>[2x]IAPLVGYAIGAAAISAVGGIGVGWTLREFEVVGSDDPAEGLTPDVLRNQLSDSVVKRKSNNQSTMVDNQNILDGVEHTAYTEAKIAAIEELNAGSSESAVLSAANSAIDSYETTVRTNFYKSWNETVRELEAMTQTVIAHADVGLSYITDFGDPRFGNLASGTSPNTLKDTTVSMPDGTNFTLLTFRHNTGWDSGNAAYSVVEYNPKEVVTSTNSNTYNTVDGTQYMKFSEWNAVETEMDTVFQNVRNGISTWVTNVYGDVQSGAIEISDLVTPRERATMMAQEEGMSQAIADLIALNVPVDAEREATITIQDTGATLPGTFALTDSSDGPLSAGQTYDPSTFSGDVYFTADMSLVEGPWDAINSGVDGGTITITSEPYEGTAIEVTTVESETVSVPAADWTDNGDGTWSYDASGDLETTITNVDSARFVSTATETTYDTLQLKGAFTVDKLVNKQSGEEVSSTSFTSSEPQTDSNYITQDEWDQLEQQNKELIEKYEQSQSGGGLDLGGLD

Haloarchaeal pleomorphic viruses (HRPVs) infect archaeal hosts living in hypersaline environments. The virions contain two major protein species, a spike protein (VP4 and VP4-like proteins) protruding from the membrane surface and a smaller membrane associated protein (VP3 and VP3-like proteins) residing mostly inside the virion. Here we describe crystallographic structures of VP4-like spike proteins from two pleolipoviruses, HRPV-2 and HRPV-6, showing that these proteins have a unique fold, different from class I–III fusion proteins. VP5 is thus a bona fide fusion protein.

In order to characterize the VP4-like fusion proteins (termed VP5 in these viruses) from HRPV-2 and HRPV-6, we purified them from infection-competent virions using either detergent (HRPV-2) or protease digestion (HRPV-6). After protein purification, we determined the structures of the HRPV-2 and HRPV-6 VP5 ectodomains (residues 1-498 out of 533 residues and 9-498 out of 537 residues) at 2.5 and 2.7 Å resolution, respectively, by X-ray crystallography. The two proteins, which are 67% identical in amino acid sequence, share a highly conserved V-shaped fold (r.m.s.d. for 453 corresponding Cα atoms: 1.6 Å). Surprisingly, the entire C-terminal domain is disordered in one of the two molecules of the asymmetric unit of HRPV-6 VP5. Although there is space in the crystal lattice to accommodate this disordered domain, the bulk of adjacent molecules prevents it from adopting the same orientation with respect to the N-terminal domain seen in the other copies of VP5. It appears that the N- and C-terminal domains can flex with respect to each other in the face of crystal packing forces. Analysis of proteinase K treated HRPV-6 particles by LC-MS/MS resulted in the identification of several peptides with core sequence FGVPGEVAV representing part of the predicted C-terminal transmembrane domain. The first twenty N-terminal residues of both VP5s are hydrophobic and predicted, by several programs for analysing hydrophobic regions of proteins, to form a transmembrane helix, indicating the preference of this region to partition into membranes. Interestingly, this hydrophobic segment is shielded from the solvent in both crystal structures by the C-terminal domain. HRPV-2 and HRPV-6 VP5 proteins share an average 67% amino acid sequence identity with the N2 subdomain being the least conserved between the two spike proteins.> MGSNDYVNQMISQMTDLAKSLNVDVTELITSVTQALEALLEEYRREGRLTDQVEKMASSVALQLAAELLAQKALEEGHDKK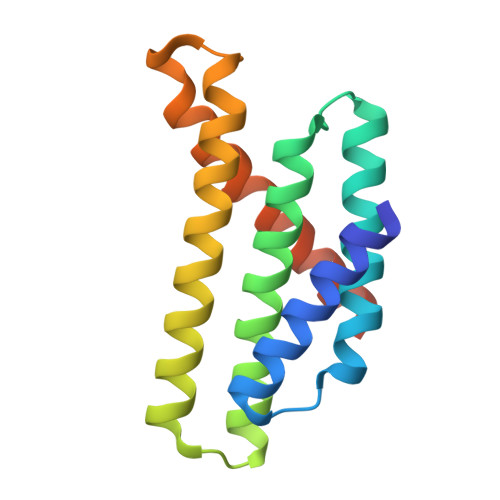QTTAKRNQISNSYSSEAMSHARAWAASRHSEEEAEKLAEELYKDMKESLKQRIDTEQVGSENLYFQ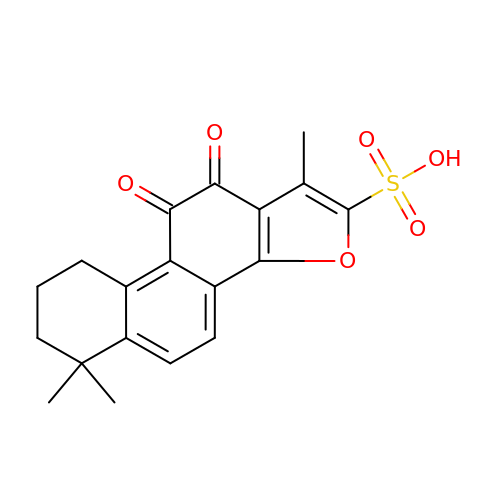1,6,6-trimethyl-10,11-dioxo-6,7,8,9,10,11-hexahydrophenanthro[1,2-b]furan-2-sulfonic acid | C19 H18 O6 S | UJCACMLMPLLRGW-UHFFFAOYSA-N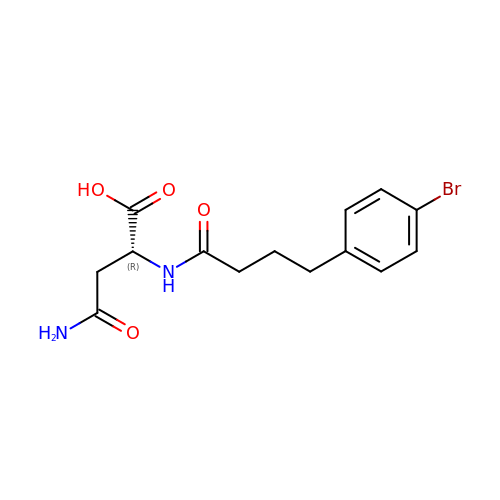N~2~-[4-(4-bromophenyl)butanoyl]-D-asparagine | C14 H17 Br N2 O4 | VRZHKETUQBKIPG-LLVKDONJSA-N> ENYLSIEKRLYENLAQESSHSASRLQFLLEHAQANTQGLSDFIGLLADKDDINNPEKLKTVLTNRIQRNPDFFGSAIAFKPNTFPNKKLFSPYVYRSGSGFNYLDIGADGYDYTDGNWDWWSKAINQVGGYWSKAYFDEGAGNVLMITYAVPFGVQPDYFGVTTVDLALDRLPEQLGIAPSRLVVLDDQGRLIFHSDKEKV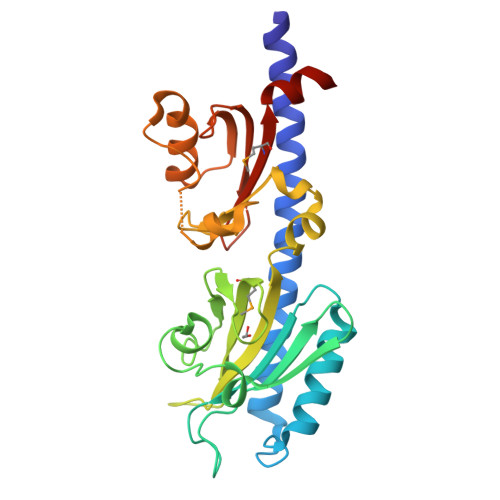LAASSSGWLDKQNIKNIAFATLLNDGQAGQASFVDDKGTVYLASVAEVAKLKWRVVVMVPKHELFASLLDDIA5-[1-[(1~{R})-1-[5-[3-chloranyl-2-fluoranyl-6-(1,2,3,4-tetrazol-1-yl)phenyl]-1-oxidanyl-pyridin-2-yl]-2-cyclopropyl-ethyl]pyrazol-4-yl]-1,3-thiazole 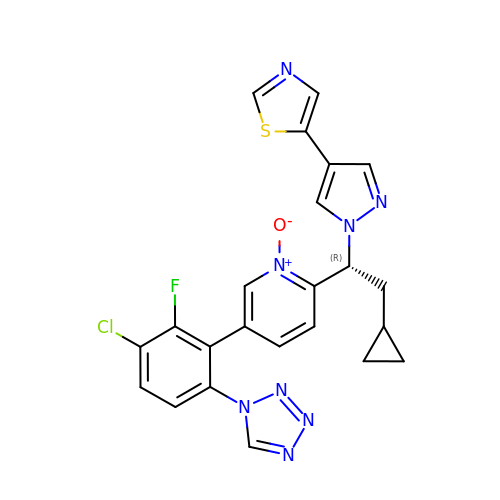| C23 H18 Cl F N8 O S | UDBRBOWRYPFBIN-HXUWFJFHSA-N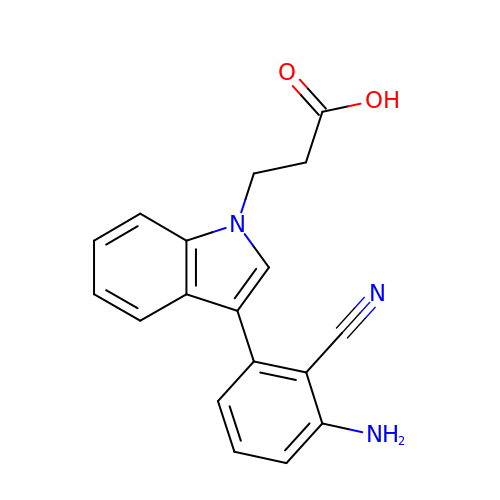3-[3-(3-azanyl-2-cyano-phenyl)indol-1-yl]propanoic acid | C18 H15 N3 O2 | BKQXGEWLSIEDTQ-UHFFFAOYSA-N>[2x]MNYKELEKMLDVIFENSEIKEIDLFFDPEVEISKQEFEDLVKNADPLQKVVGDNYITETFEWWEFENQYLEFELDYYVKDEKIFVLEMHFWRKIRKLEHHHHHH;> MRNLKRIVMGENKLIGLVRTALDSITLGQGVNEAKIKSPQSYAFHTISVGTISLDICKAIYSSSEIGRKQLENLSKKYNMPFEDLWFYGGFLHDWNKLSGKEESLENKEELTKKIIDKLKLPNEFLHGISTMAEGHLPDNLHLPLWVSIKLADMLLISDIGSVRDVFYFANSDSYRNAIEALKEYNLELNYVSSTFRLFTLIASKELLNDVFNEKSGYFPLISYADGIVFLKRKNSQPVLLSKIVDLLSRQVFSSSSEVIEEKISDIEKCIKNKEELFRQMNIDVKSAIYDEEGKVKQINAFLPTKVCKPFEDVVGNLDNKSKLQVAREVIERNRKDIPFGLLIYFVNKFSKNEEDYIRKGLGINEKSLKYLLNIGDVQKALDKILELLEKRYAEQSSDKTLLYYVKFSSSGNIIDDLPKITDRPNDYCVVCGMPIYSSNPVRFVQYASELGGRAEIWIPREKALDEIDNVRDDWKVCPICIYEANLMKDRVKPPYFIVTFYPGVPISLLNIIDFDFSQSSIKYYIDEEKDTYFTAFEKMGGRLEPYVKKVLPAYFSSKVIIKASEVSNFSLSTRLSKSELNKLLPYAPMISMIFLTSPVLISSNLYEMPIAHERVISITSTYNYTFMKSLNSNLLTLYSIFAYSAKYDAMRKICGRSDLDNCLGYLTEEMDLYSSVDPALGVLSIGMGVGTPIDTDEKFFSAFLPVSGYLLKVTGKVSKMGETLKSSIFSIAYALKDIIKSQKVSKYDVTGFLRDGVDMFFKTTSVIKDKEDRIGISVNAAISSLENKYALDDQHRAQVYSALQDIFKTLYSIEEESDRSLAISIANTLSNWLYIAYKLVLQGDKSLEHHHHHH

Type I-D CRISPR–Cas systems, which are found both in bacteria and archaea, are exceptional in that they contain a hybrid large subunit, Cas10d, bearing resemblance to both the signature proteins found in type I (Cas3) and type III (Cas10). Here, we present the crystal structure of the Cas10d large effector complex subunit from the Sulfolobus islandicus I-D system, both in isolation and in complex with the Sulfolobus islandicus rod-shaped virus 3 (SIRV3) anti-CRISPR protein, AcrID1. As predicted from comparative sequence analysis, the 847 residue (94 kDa) S. islandicus Cas10d consists of six domains: A HD nuclease domain (1–186), a Cyclase/RRM domain (187–425), a zinc finger domain (426–490), a Palm/RRM domain (491–623), and a C-terminal helical region consisting of a polymerase-like Thumb domain (624–719) and an extension with predicted homology to Cas11 (720–847). In this paper, we demonstrate that the S. islandicus type I-D large subunit, Cas10d, has a unique structure consisting of a type I-like HD nuclease domain joined to a set of inactivated type III-like nucleotidyl transferase domains and a Cas11-like C-terminal domain.

To understand the molecular architecture of the unique type I-D system as well as mechanism of inhibition by AcrID1, we reconstituted the Cas10d–AcrID1 complex in vitro and determined the crystal structure to 3.5 Å resolution by single-wavelength anomalous dispersion (SAD) phasing using Se–Met substitution. The net result of these interactions is that two AcrID1 dimers sequester two Cas10d subunits into a large, circular 4:2 complex. The buried surface areas between the AcrID1 dimer and the two molecules of Cas10d constitute approximately 930 and 880 Å2 at the two distinct sites of interaction, and size exclusion chromatography supports that this higher-order complex represents the biologically relevant form. In the 2:4 complex of Cas10d and AcrID1 there are no direct interactions between the two Cas10d subunits but several specific interactions between both AcrID1 monomers and each domain of Cas10d that effectively cross-link the Cas10d subunits. These interactions tie one AcrID1 monomer (chain A) to the HD nuclease, Palm/RRM, and Thumb/Cas11 domains of one Cas10d subunit and the other AcrID1 monomer (chain B) to the Cyclase/RRM and C-terminal Thumb domains of another Cas10d subunit. Contacts to the Cyclase/RRM domain are extensive and involve both charged and hydrogen bond interactions to two exposed loops (273–275 and 292–307). The interactions between AcrID1 and the HD nuclease domain are especially intriguing because they involve an N terminal extension of Cas10d (residues 1–13) for which specific contacts are made to both Asn3 and Arg6.>HHHHHHFNLPPGNYKKPVLLYTSNGGHFLRILPDGTVDGTRDRSDQHIQLQLSAESVGEVYIKSTETGQYLAMDTDGLL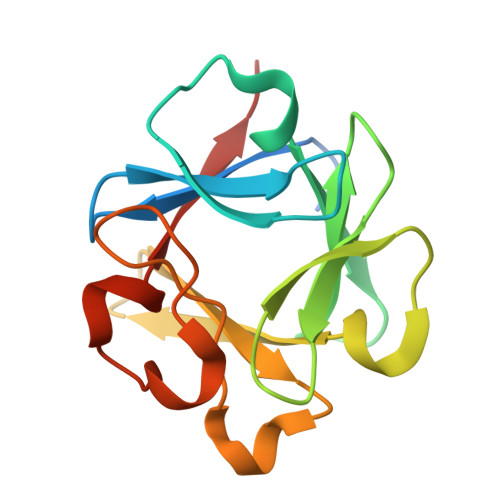YGSQTPNEECLFLERLEENHYNTYISKKHAEKNWFVGLKKNGSVKRGPRTHYGQKAILFLVLPVSSD[2x]>[2x]GLFDIIKKVASVIGGL

Citropin 1.3 is an antimicrobial peptide secreted by the amphibian Litoria citropa (Southern bell frog). In this study, the structural and functional properties of its non‐amidated form, which self‐assembles into distinct fibrillar architectures, are investigated. Using cryogenic electron microscopy, X‐ray crystallography, and fluorescence microscopy with model membranes and cells, diverse supramolecular structures, including canonical amyloid fibrils, multilayered nanotubes, and a novel mixed fibril type, are identified. Citropin 1.3 with free, charged termini, has a net positive charge of +1 at neutral pH, primarily consists of hydrophobic residues (9 out of 16 residues) and adopts an amphipathic α‐helical structure in its monomeric form.

Citropin 1.3 was found to form cubic microcrystals, which diffracted to a resolution of 1.6 Å. The crystal structure revealed two chains of the 16‐residue peptide within the asymmetric unit. These peptide chains adopt α‐helical conformations, tightly packed through hydrophobic interactions involving residues such as Ile5, Val9, Val12, and Leu16. Additionally, a hydrogen bond is formed between Lys8 on chain B and Ser11 on chain A. Each chain also exhibits an internal electrostatic interaction between Lys8 and Asp4. The α‐helical dimers further assemble into a spiraling supramolecular structure. Inter‐dimer interactions include tight packing between Phe3 and Lys7 of neighboring chain Bs, alongside interactions with Leu16 from chain A. Furthermore, Ala10 and Ile13 from chains A and B of adjacent dimers engage in hydrophobic packing, as do Leu2 and Ile5 from neighboring A chains. These tightly packed helices collectively form a supramolecular assembly resembling a nanotube. The fibril's surface features alternating hydrophobic and positively charged zigzagged belts. Nonetheless, the structure confirms that citropin 1.3 can adopt α‐helical conformations in addition to the β‐strand‐rich structures observed in cryo‐EM studies.>VIHNESTCEQLAKANAGKPKDPTFIPAPIQAKTSPVDEKALQDQLVLVAAKLDTEDKLRAAMVGMLANFLGFRIYGMHSELWGVVHGATVLSPTAVFGTLASLYLGALDHTADRLQAILGVPWKDKQCTSRLDAHKVLSALQAVQGLLVAQGRADSQAQLLLSTVVGVFTAPGLHLKQPFVQGLALYTPVVLPRSLDFTELDVAAEKIDRFMQAVTGWKTGSSLMGASVDSTLAFNTYVHFQGKMKGFSLLAEPQEFWVDQSTSVSVPMLSGMGTFQHWSDIQDQFSVTQVPFTESASLLLIQPHYASDLDKVEGLTFQQNSLNWMKKLSPRTIHLTMPQLVLQGSYDLQDLLAQA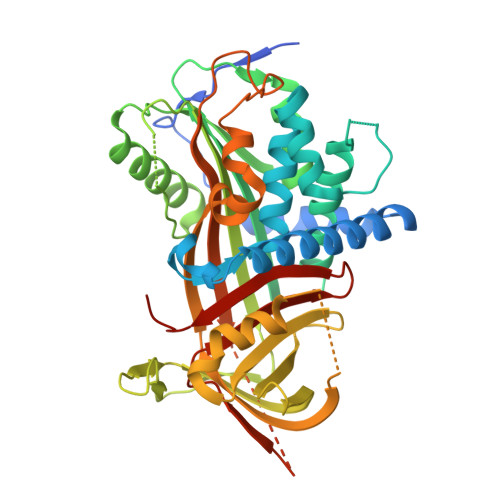ELPAILHTELNLQKLSNDRIRVGEVLNSIFFELEADEREPTESTQQLNKPEVLEVTLNRPFLFAVYDQSATALHFLGRVANPLSTAHHHHHH[2x]>[4x]XIE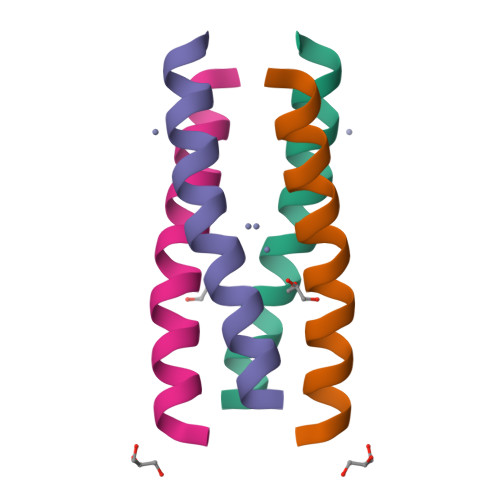ELLRKILEDDARHVAELEDIEKWLX>[8x]SDGTVIDLATITKNITDAVAFAKSVKDVHTLVKSIDELAKAIGKKIGANGLETDADKNAKLISGAYSVISAVDTKLASLEKKVGISDDLKGKITT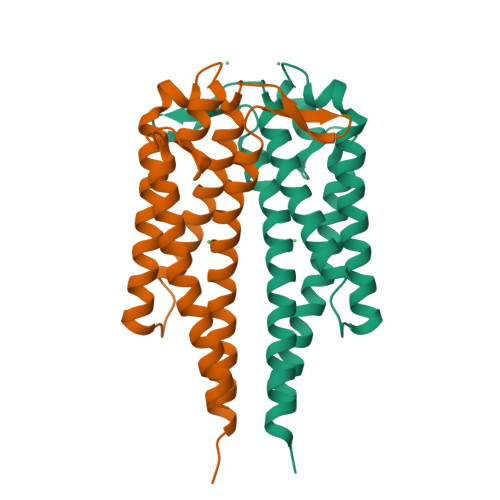VKNASTSFLTKAKSKTADLGKDDVKDADAKTAIDIADTGAKDKGAEELIKLNTAIDALLTSAEAAVTAAINALSTPAKSASTVQSN N-[2-(4-AMINO-5,8-DIFLUORO-1,2-DIHYDROQUINAZOLIN-2-YL)ETHYL]-3-FURAMIDE | C15 H14 F2 N4 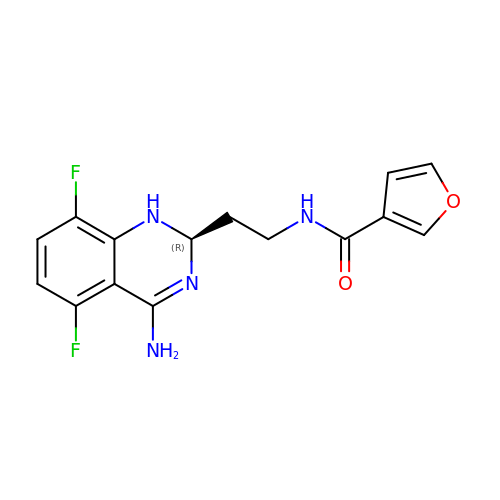O2 | BOAUWUUBSXECNL-LLVKDONJSA-N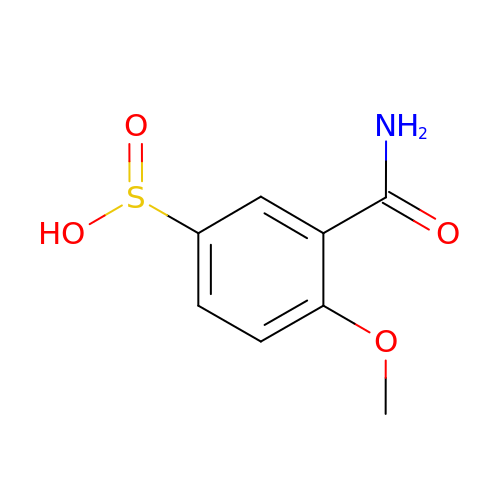(S~1~R)-3-carbamoyl-4-methoxybenzene-1-sulfinic acid | C8 H9 N O4 S | ORKHLRISPIOULZ-UHFFFAOYSA-N> WSHPQFEKENLYFQSPRLLSHCGRAAHCEPLRYNVCLGSALPYGATTTLLAGDSDSQEEAHGKLVLWSGLRNAPRCWAVIQPLLCAVYMPKCENDRVELPSRTLCQATRGPCAIVERERGWPDFLRCTPDHFPEGCPNEVQNIKFNSSGQCEAPLVRTDNPKSWYEDVEGCGIQCQNPLFTEAEHQDMHSYIAAFGAVTGLCTLFTLATFVADWRNSNRYPAVILFYVNACFFVGSIGWLAQFMDGARREIVCRADGTMRFGEPTSSETLSCVIIFVIVYYALMAGVVWFVVLTYAWHTSFKALGTTYQPLSGKTSYFHLLTWSLPFVLTVAILAVAQVDGDSVSGICFVGYKNYRYRAGFVLAPIGLVLIVGGYFLIRGVMTLFSIKSNHPGLLGIDCSFWNESYLTGSRDERKKSLLSKFGMDEGVTFMFIGRFDRGQKGVDVLLKAIEILSSKKEFQEMRFIIIGKGDPELEGWARSLEEKHGNVKVITEMLSREFVRELYGSVDFVIIPSYFEPFGLVALEAMCLGAIPIASAVGGLRDIITNETG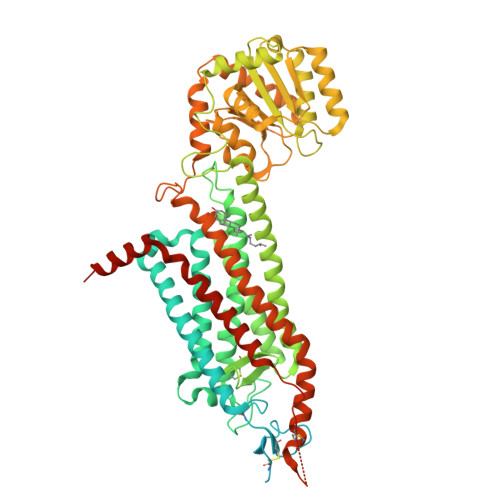ILVKAGDPGELANAILKALELSRSDLSKFRENCKKRAMSFSDQARMDIRLAKNETMLRLGIFGFLAFGFVLITFSCHFYDFFNQAEWERSFRDYVLCQANVTIGLPTKKPIPDCEIKNRPSLLVEKINLFAMFGTGIAMSTWVWTKATLLIWRRTWCRLTGHSDDEPKR> PEIVDTCSLASPASVCRTKHLHLRCSVDFTRRTLTGTAALTVQSQEDN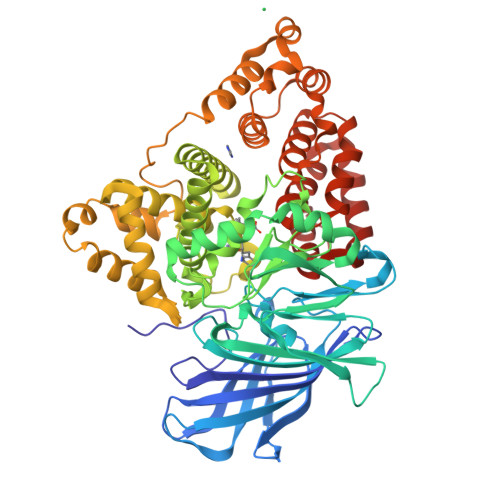LRSLVLDTKDLTIEKVVINGQEVKYALGERQSYKGSPMEISLPIALSKNQEIVIEISFETSPKSSALQWLTPEQTSGKEHPYLFSQCQAIHCRAILPCQDTPSVKLTYTAEVSVPKELVALMSAIRDGETPDPEDPSRKIYKFIQKVPIPCYLIALVVGALESRQIGPRTLVWSEKEQVEKSAYEFSETESMLKIAEDLGGPYVWGQYDLLVLPPSFPYGGMENPCLTFVTPTLLAGDKSLSNVIAHEISHSWTGNLVTNKTWDHFWLNEGHTVYLERHICGRLFGEKFRHFNALGGWGELQNSVKTFGETHPFTKLVVDLTDIDPNVAYSSVPYEKGFALLFYLEQLLGGPEIFLGFLKAYVEKFSYKSITTDDWKDFLYSYFKDKVDVLNQVDWNAWLYSPGLPPIKPNYDMTLTNACIALSQRWITAKEDDLNSFNATDLKDLSSHQLNEFLAQTLQRAPLPLGHIKRMQEVYNFNAINNSEIRFRWLRLCIQSKWEDAIPLALKMATEQGRMKFTRPLFKDLAAFDKSHDQAVRTYQEHKASMHPVTAMLVGKDLKVD> MGMPVPGTLSVEIPPRYCPLPTARHPDETVLARRTADWIDGFDLELTPQQRARMRGNDAPGFYGRIMPHSPTDRLQLAVDWCTVMFHFDDVHCDEGPATGRAARFADLATRIVRVLEAPDARLEGPGDTMLAPVRDLALRARRWATPAQMRRCAEAHRAWFLAVAWELGHRAARSTPALNDYAHMRQHTAAGAATLAWAEIVDGAEIPDRELSSPEVRALTELAFTTAAFDDDLFSYGKELWVARAEGTAPSGLGLVEILRRENRCGRPEALRAAVCLCNRLTHRFIALRERVLPDASAPLRAYLDHLCHLLPGNLEWGLTADRYRNPDGRTPGAVTTTASRDTDPPADTSPPAIPSIAWWWDPLGGRPATEHHHHHH

We recently discovered the cattleyene synthase (CyS) from Streptomyces cattleya and studied its cyclization mechanism through isotopic labelings. Some polycyclic diterpenoids have attracted increasing attention, e.g. gibberellins are phytohormones derived from ent‐kaurene, while phorbol esters exhibiting the tigliane skeleton are currently in phase II clinical trials for the treatment of acute myeloid leukemia. Their biosynthesis is attributed to diterpene synthases (DTSs), the type I of which catalyzes the conversion of GGPP through diphosphate abstraction and cationic cascade reactions. Substrate ionization is mediated by a Lewis acidic trinuclear Mg2+ cluster, bound itself to a highly conserved Asp‐rich motif (DDXX(X)D) and an NSE/DTE triad ((N,D)DLX(S,T)XXXE), to which the substrate's pyrophosphate docks, with assistance of a highly conserved Arg residue (pyrophosphate sensor). Here we report on the crystal structures of apo‐CyS, CyS complexed with GGPP and Mg2+ (CyS‐GGPP‐Mg2+), and the CySC59A enzyme variant.

For a deeper understanding of the increased but less selective production by the C59A variant (CysC59A), its crystal structure was solved at 2.30 Å. The structure is highly similar to the apo‐CyS and CyS‐GGPP‐Mg2+ structures (RMSD of 0.16 Å and 0.15 Å for Cα atoms). The active site residues of the three structures superimpose well, with the exception of F86 located between C59 and the substrate binding pocket. In the apo‐CyS and CyS‐GGPP‐Mg2+ structures, the thiol of C59 is close to the phenyl ring of F86 (3.4 Å) and renders it towards the active site, while in CySC59A this interaction is disrupted. As a result, F86 moves a bit away from the active site and the phenyl ring rotates 24° clockwise. This slightly widens the active site cavity which may lead to an improved uptake of GGPP, albeit on the expense of selectivity because of a less tight substrate control through cation‐π interactions. Gratifyingly, the C59A variant gave a similar product profile, but with a much better production (about 6‐fold in comparison to the F86A variant except for 3). The C59A exchange widens the active site cavity, resulting in a relaxed product selectivity, with a series of unprecedented ring closures and skeletal rearrangements towards 6. However, such alignment based targetings cannot fully substitute for the structure based identification of residues, and in fact the position analogous to C59 in CyS has not been targeted in any other TS before. For this purpose, all 20 isotopomers of (13C)GGPP, prepared enzymatically from 13C‐labeled FPP, GPP or IPP precursors, were enzymatically converted with CySC59A, followed by extraction with C6D6 and analysis of the product mixture through 13C NMR.>[4x]TPYMVQPEYRI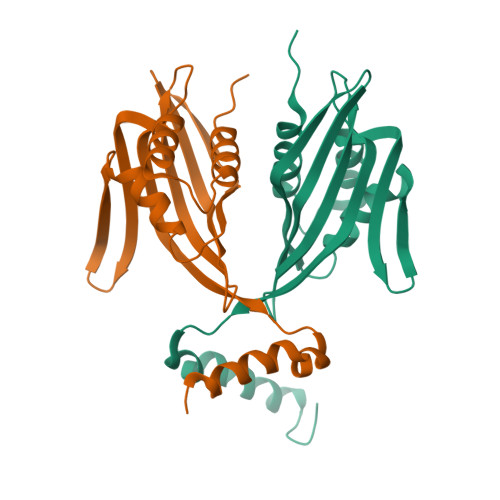YEMNKRLQSRTEDSDNLWWDAFATEFFEDDATLTLSFCLEDGPKRYTIGRTLIPRYFSTVFEGGVTDLYYILKHSKESYHNSSITVDCDQCAMVTQHGKPMFTKVCTEGRLILEFTFDDLMRIKTWHFTIRQYRELVPRSILAMHAQDPQVLDQLSKNITRMGLTNFTLNYLR> DDIPDMEEFD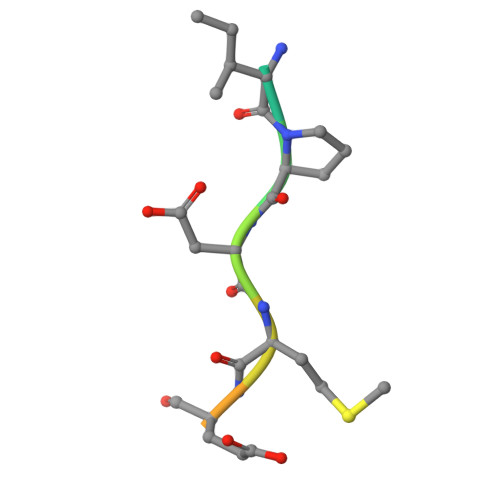E>[4x]MPQDVVFDLPWPLRKHPGVAGAREHCLGWLAA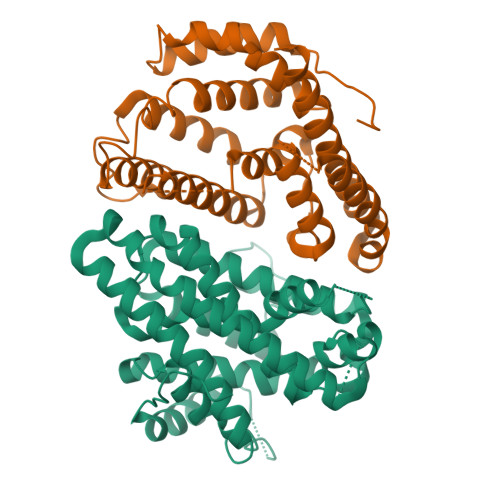QGLADRRGLTAETFVTWQLDELAGYFFPRATQEGLELATDLMVWYFAPFDDQFDGALGRDPRRTAGVCAGLAEVLYGVPEPGPVASSPVGRALGDLWRRSCTGMSPFWRTRARHNWTGYLAAHTAESVPRYHGRTVDAAYCVRQRGYATSSHVIMDLIERTGGFEVPAMVWHHPVLVELRTLTSEMIGISNDLCSAEKEEADGDLSNNLLLVLENHEGLDRPEAIERARALTAERVARFLDVERAVTDVDCLLDGAGREAVRRFVEGLHDLVRGDNEWERTTGRYQPAISGLQDLADLMSSGWDPLASGTAAGHGGHTR> GSHMKNSVSVDLPGEMKVLVSKEKNKDGKYDLIATVDKLELKGTSDKNNGSGVLEGVKADKSKVKLTISDDLGQTTLEVFKEDGKTLVSKKVTSKDKSSTEEKFNEKGELSEKKITRADKSSTEEKFNEKGELSEKKITRADKSSTEEKFNEKGELSEKKITRADKSSTEEKFNEKGEVSEKIITRADGTRLEYTGIKSDGSGKAKEVLKGYVLEGTLTAEKTTLVVKEGTVTLSKNISKSGEVSVELNDTDSSAAT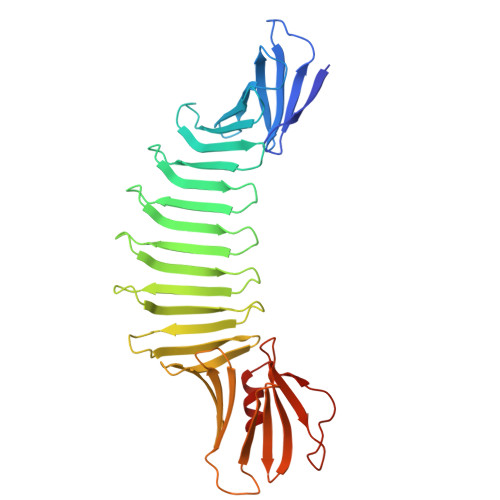KKTAAWNSGTSTLTITVNSKKTKDLVFTKENTITVQQYDSNGTKLEGSAVEITKLDEIKNALK>[2x]GPLGSM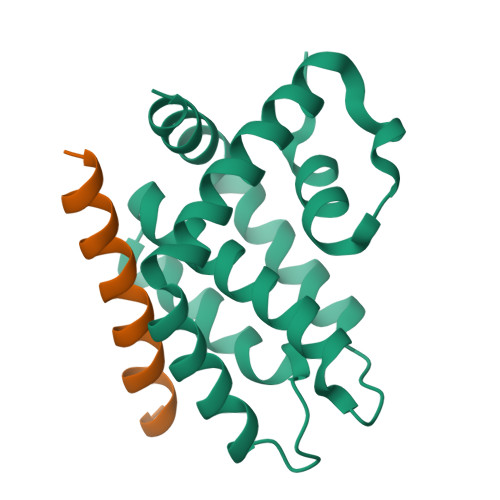DNCNYNIEKVLNVYLRDLRIESLNNNELEILIMIRECCEVIKKDYKTEFNEICNFILQNNVKSCYDINDVKNIIIETINSDFRPSVILASISLLSIIIKKKKDENNEVVDDDLALNELINKFSSYQKDIISFVEKNKKKNKQND;>VPQDASTKKLSECLKRIGDELDSNMELQ[8x];>[6x]MDNCNYNIEKVLNVYLRDLRIESLNNNELEILIMIRECCEVIKKDYKTEFNEICNFILQNNVKSCYDINDVKNIIIETINSDFRPSVILASISLLSIIIKKKKDENNEVVDDDLALNELINKFSSYQKDIISFVEKNKKKNKQND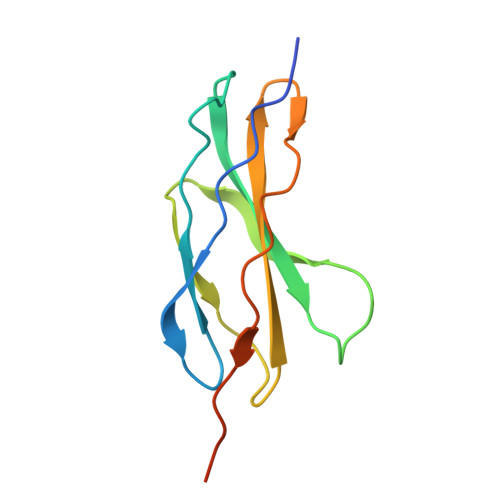> AEPSSPPGAPSQPVVTEITKNSITLTWKPNPQTGAAVTSYVIEAFSPAAGNTWRTVADGVQLETHTVSGLQPNTIYLFLVRAVGAWGLSEPSPVSEPVRTQDSSPSRPVEDPWR>[4x]SNAMHMLRIAKEALTFDDVLLVPAHSTVLPNTADLRTRLTKNIALNIPMVSASMDTVTEARLAIALAQEGGIGFIHKNMSIEQQAAQVHQVKISGGLRVGAAVGAAPGNEERVKALVEAGVDVLLIDSSHGHSEGVLQRIRETRAAYPHLEIIGGNVATAEGARALIEAGVSAVKVGIGPGSICT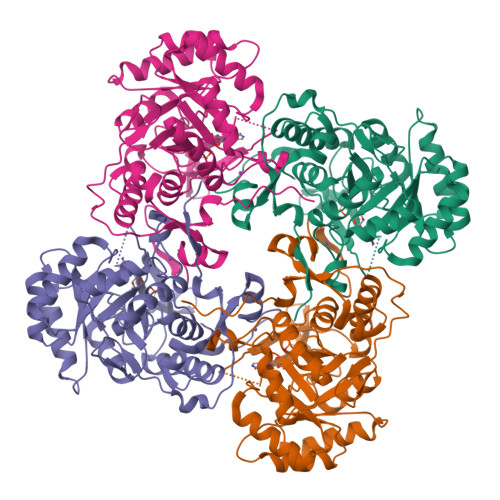TRIVTGVGVPQITAIADAAGVANEYGIPVIADGGIRFSGDISKAIAAGASCVMVGSMFAGTEEAPGEVILYQGRSYKAYRGMGSLGAMSKGSSDRYFQTDNAADKLVPEGIEGRIAYKGHLKEIIHQQMGGLRSCMGLTGSATVEDLRTKAQFVRISGAGMKESHVHDVQITKEAPNYRLG> MFKIGSVLKQIRQELNYHQIDLYSGIMSKSVYIKVEADSRPISVEELSKFSERLGVNFFEILNRAGMNTKSVNETGKEKLLISKIFTNPDLFDKNFQRIEPKRLTSLQYFSIYLGYISIAHHYNIEVPTFNKTITSDLKHLYDKRTTFFGIDYEIVSNLLNVLPYEEVSSIIK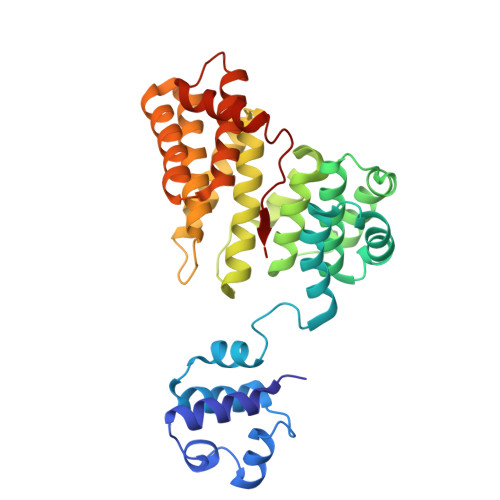PMYPIVDSFGKDYDLTIQTVLKNALTISIMNRNLKEAQYYINQFEHLKTIKNISINGCYDLEINYLKQIYQFLTDKNIDSYLNAVNIINIFKIIGKEDIHRSLVEELTKISAKEKFTPPKEVTMYYENYVAIENNPIPEIKEQS Condensin I is a multi‐protein complex that plays an essential role in mitotic chromosome assembly and segregation in eukaryotes. It is composed of five subunits: two SMC (SMC2 and SMC4), a kleisin (CAP‐H), and two HEAT‐repeat (CAP‐D2 and CAP‐G) subunits. SMC2 and SMC4 dimerize through their hinge domains to form a V‐shaped heterodimer, and CAP‐H, which belongs to the kleisin family of proteins, bridges SMC head domains through its C‐ and N‐terminal regions. CAP‐D2 and CAP‐G, both of which are composed of arrays of short amphiphilic helices known as HEAT repeats, bind to the central region of CAP‐H 4, 5.

As the most C‐terminally located motif V was predicted to bind to SMC2 21, we thought that motif IV (residues 461–503) may be responsible for binding to hCAP‐G. With this information, we aimed to express and purify hCAP‐G complexed with a fragment of hCAP‐H. We found that the N‐terminal domain of hCAP‐G (residues 1–478) connected to the C‐terminal domain of hCAP‐G (residues 554–900), and a fragment of hCAP‐H containing motif IV (residues 460–515) was able to be co‐expressed and co‐purified. This hCAP‐G‐H subcomplex was successfully crystalized and its structure was determined at 3.0 Å resolution. Two molecules of the hCAP‐G‐H subcomplex are present in the crystallographic asymmetric unit (Fig EV2A). Their structures are essentially identical, but 4‐(2‐hydroxyethyl)‐1‐piperazineethanesulfonic acid (HEPES) is bound to only one of the two molecules. In the current report, we describe the HEPES‐bound hCAP‐G‐H subcomplex (a, b‐molecules) as a representative structure. Consistent with the recent assignment based on its amino acid sequence 5, hCAP‐G displays a “harp‐shaped” structure composed of 19 HEAT repeats (H1‐H19), in which H12 and H15 have long disordered loops (residues 479–553 and 661–691, respectively) (Figs 1C and EV1A and EV2B). hCAP‐H, which comprises three α‐helices (α2, α3′, and α4), binds to the concave surfaces of hCAP‐G (Figs 1C and EV1B). Second, hCAP‐H is more loosely bound to hCAP‐G than the yeast counterpart, resulting in the more opened conformation of the HEAT‐repeat subunit hCAP‐G. The distance between R257 and V754 of hCAP‐G is 17.06 Å, whereas the corresponding distance between R287 and F749 of YCG1 is 6.25 Å (Fig EV3A). The previous electron microscopy study also demonstrated that the HEAT‐repeat subunit of cohesin loader, Scc2, adopted several flexible conformations. These observations of the structural flexibility led us to speculate that our hCAP‐G‐H structure represents a snapshot of an “open conformation”, whereas the structure of its yeast counterpart represents a snapshot of a “closed conformation”. hCAP‐H interacts extensively with the concave surface of hCAP‐G at four major sites, whereas YCG1 interacts with BRN1 at five major sites (Fig EV3A) 17. At site IV, there are notable hydrogen bonds formed between H512 and L513 of hCAP‐H and D647 of hCAP‐G.

>MEIDFEDDIDFDVYFRKTKAATILTKSTLENQNWRATTLPTDFNYNVDTLVQLHLKP[2x];>[2x]MGSSHHHHHHSQDPMGAERRLLSIKEAFRLAQQPHQNQAKLVVALSRTYRTMDDKTVFHEEFIHYLKYVMVVYKREPAVERVIEFAAKFVTSFHQSDMEDDEEEEDGGLLNYLFTFLLKSHEANSNAVRFRVCLLINKLLGSMPENAQIDDDVFDKINKAMLIRLKDKIPNVRIQAVLALSRLQDPKDDECPVVNAYATLIENDSNPEVRRAVLSCIAPSAKTLPKIVGRTKDVKEAVRKLAYQVLAEKVHMRAMSIAQRVMLLQQGLNDRSDAVKQAMQKHLLQGWLRFSEGNILELLHRLDVENSSEVAVSVLNALFSITPLSELVGLCKNNDGRKLIPVETLTPEIALYWCALCEYLKSKGDEGEEFLEQILPEPVVYADYLLSYIQSIPVVNEEHRGDFSYIGNLMTKEFIGQQLILIIKSLDTSEEGGRKKLLAVLQEILILPTIPISLVSFLVERLLHIIIDDNKRTQIVTEIISEIRAPIVTVGVAETLQKCLILCYELLKQMSISTGLSATMNGIIESLILPGIISIHPVVRNLAVLCLGCCGLQNQDFARKHFVLLLQVLQIDDVTIKISALKAIFDQLMTFGIEPFKTKKIKTLHCEGTEINSDDEQESKEVEETATAKNVLKLLSDFLDSEVSELRTGAAEGLAKLMFSGLLVSSRILSRLILLWYNPVTEEDVQLRHCLGVFFPVFAYASRTNQECFEEAFLPTLQTLANAPASSPLAEIDITNVAELLVDLTRPSGLNPQAKTSQDYQALTVHDNLAMKICNEILTSPCSPEIRVYTKALSSLELSSHLAKDLLVLLNEILEQVKDRTCLRALEKIKIQLEKGNKE>MVSASQRTTSTATGDEWWAKCKQVDVLDSEMSYYDSDPGKHKNTVIFLHGNPTSSYLWRNVIPHVEPLARCLAPDLIGMGKSGKLPNHSYRFVDHYRYLSAWFDSVNLPEKVTIVCHDWGSGLGFHWCNEHRDRVKGIVHMESVVDVIESWDEWPDIEEDIALIKSEAGEEMVLKKNFFIERLLPSSIMRKLSEEEMDAYREPFVEPGESRRPTLTWPREIPIKGDGPEDVIEIVKSYNKWLSTSKDIPKLFINADPGFFSNAIKKVTKNWPNQKTVTVKGLHFLQEDSPEEIGEAIA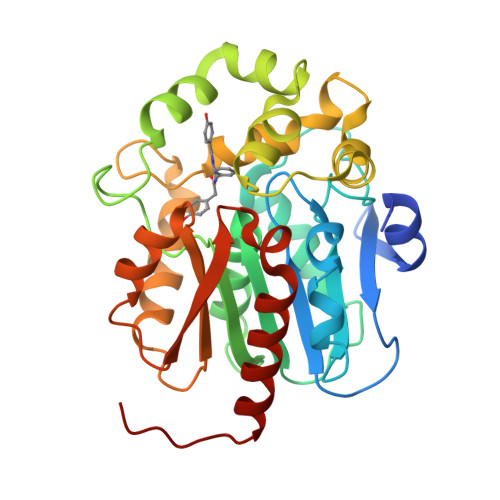DFLNELTKHHHHHH[3x]>[3x]GSHMASMFGKLREKLKSFVKRVEEEVEKEEEEVEKKGLLDRILTVEIKEKDVDKALDELEIDLLEADVALEVVDALREKIKQKLVGKKVRIGTDKGKIIEEAVKEAVSEILETSRRIDLIEEIRKAEKPYVIMFVGFNGSGKTTTIAKLANWLKNHGFSVVIAASDTFRAGAIEQLEEHAKRIGVKVIKHSYGADPAAVAYDAIQHAKARGIDVVLIDTAGRSETNRNLMDEMKKIARVTKPNLVIFVGDALAGNAIVEQARQFNEAVKIDGIILTKLDADARGGAALSISYVIDAPILFVGVGQGYDDLRPFEKEWFLERIFGEENA

The process is mediated by evolutionarily related signal recognition particles (SRPs) and their cognate membrane-associated receptors (SRs also called FtsYs in Bacteria and Archaea). The core proteins of SRPs and SRs are GTPases that each contain a structurally and functionally conserved NG domain where the G domain adopts a ras-like fold responsible for GTP binding and the N-domain adopts a four α-helix bundle fold. Here we describe the X-ray structures and solution conformations of FtsY, the SR from the hyper-thermophilic archaeon Pyrococcus furiosus (Pfu), in its free and GDP•magnesium-bound forms. The low resolution, solution scattering data complements our high-resolution crystallographic analysis and shows that the crystallographic structure and the average conformation adopted in solution are similar. While the overall architecture of the archeal receptor resembles its previously described bacterial homologues from the SRP/SR GTPases family, the structure of Pfu-FtsY reveals novel features: The elongated N domain lacks the N-terminal extension observed in all other bacterial FtsYs and is instead characterized by a long N-terminal helix αN1 that packs against the NG core in a different way; sequence analysis suggests that archeal receptors may cluster apart from their bacterial homologues.

The apo receptor was crystallized in two different crystallization conditions in absence of guanine nucleotide and its structure solved de novo using single wavelength anomalous dispersion of selenium; the structure is therefore not biased towards any of the previously solved homologues. Our Pfu-FtsY structure is the first representative from the Archaea kingdom. The Pfu-FtsY construct used in this study encodes the full-length receptor. The αN1 helix of Pfu-FtsY is not bent and its axis is shifted towards the core of the four α-helix bundle resulting in an overall more compact, albeit extended, N domain. In Pfu-FtsY, the N-terminus of helix αN1 is positively charged and could constitute the primary membrane interaction site supporting initial attachment of the targeting complex to the membrane and/or interaction with the membrane-embedded translocon.(3R,4S)-1-[(4-amino-5H-pyrrolo[3,2-d]pyrimidin-7-yl)methyl]-4-{[(4-chlorophenyl)sulfanyl]methyl}pyrrolidin-3-ol | C18 H20 Cl N5 O S | 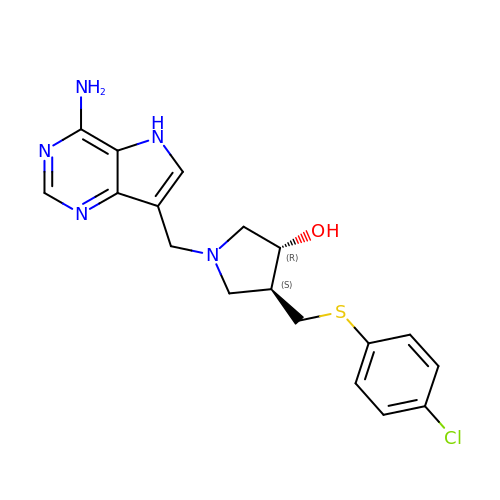MZZBHZOHYGEGEE-DOMZBBRYSA-N> GIILTKVGYYTIPSMDDLAKITNEKGECIVSDFTIGRKGYGSIYFEGDVNLTNLNLDDIVHIRRKEVVVYLDDNQKPPVGEGLNRKAE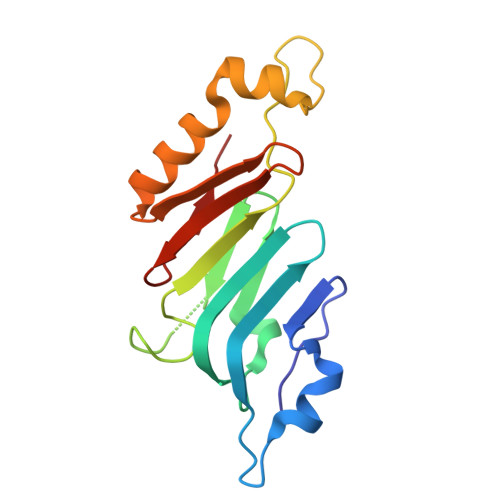VTLDGVWPTDKTSRCLIKSPDRLADINYEGRLEAVSRKQGAQFKEYRPETGSWVFKVSHFAKYGLQD> MKQYLELMQKVLDEG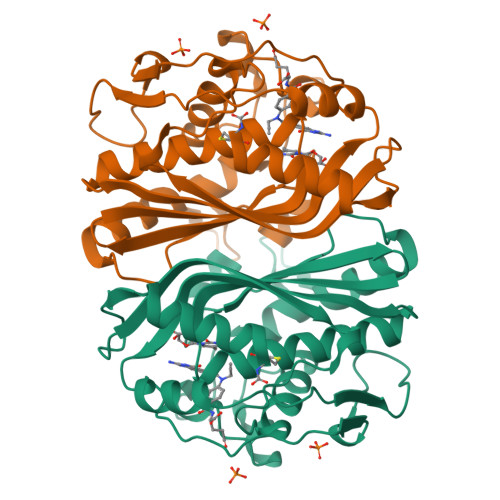TQKNDRTGTGTLSIFGHQMRFNLQDGFPLVTTKRCHLRSIIHELLWFLQGDTNIAYLHENNVTIWDEWADENGDLGPVFGKQWRAWPTPDGRHIDQITTVLNQLKNDPDSRRIIVSAWNVGELDKMALAPCHAFFQFYVADGKLSCQLYQRSCDVFLGLPFNIASYALLVHMMAQQCDLEVGDFVWTGGDTHLYSNHMDQTHLQLSREPRPLPKLIIKRKPESIFDYRFEDFEIEGYDPHPGIKAPVAI> GSH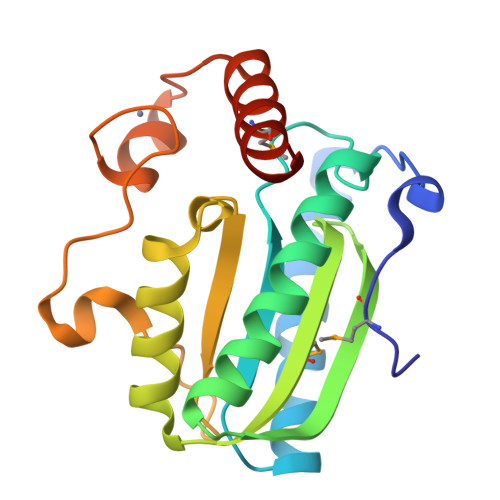MHLLPELASHHAVSIPELLVSRDERQARQHVWLKRHPVPLVSFTVVAPGPIKDSEVTRRIFNHGVTALRALAAKQGWQIQEQAALVSASGPEGMLSIAAPARDLKLATIELEHSHPLGRLWDIDVLTPEGEILSRRDYSLPPRRCLLCEQSAAVCARGKTHQLTDLLNRMEALLNDVDACNVN>[2x]MSLNKQDGENTLQHEKSSSFGYWCSPSPEQLERLSLKQLAAVSNFVIGRRGYGCITFQHDVDLTAFTKSFREELFGKIVIFRSSK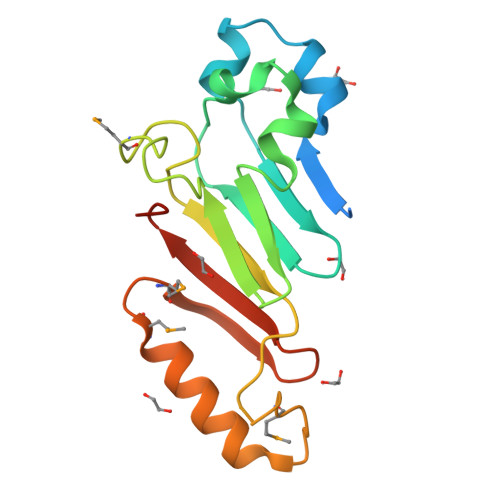TVEVYPDEATKPMIGHGLNVPAIITLENVYPVDKKTKKPMKDTTKFAEFQVFDRKLRSMREMNYISYNPFGGTWTFKVNHFEGHHHHHH> MNVRFRRRFLTAALAAVAVAAAPAVHAQAAGKPKVALVMKSLANEFFLTMENGAKEYQKHNASQFDLITNGIKDETDTANQIRIVEQMIVSKVDAIVLAPADSKALVPVVKKAVDAGIIVVNIDNRLDPD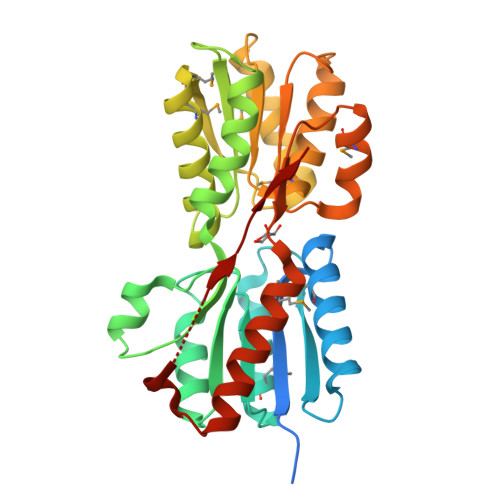VLKSKNLNVPFVGPDNRKGARKVGDYLAKKLKAGDQVGIVEGVSTTTNAQQRTAGFQDAMKAGGMKVVSVQSGEWEIDKGNAVASAMLNEYPNLKALLCGNDNMAIGAVSAVRAAGKQGKVYVVGYDNINAIKPMLKDGRVLATADQYAAKQAVFGIDTALKAIAEHRKQAELSGVVETPVDLVTK>MIIREATVQDYEEVARLHTQVHEAHVKERGDIFRSNEPTLNPSRFQAAVQGEKSTVLVFVDEREKIGAYSVIHLVQTPLLP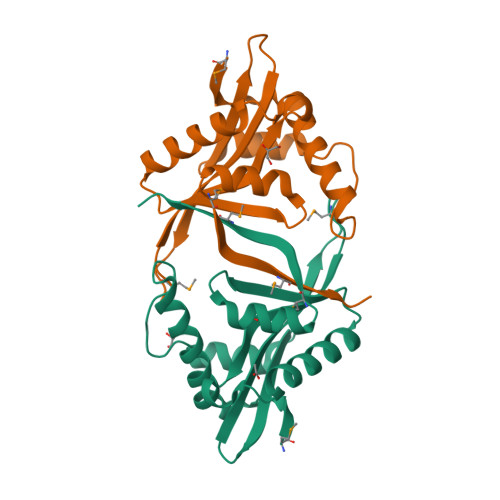TMQQRKTVYISDLCVDETRRGGGIGRLIFEAIISYGKAHQVDAIELDVYDFNDRAKAFYHSLGMRCQKQTMELPLLEHHHHHH[2x]>GSSGAFEDRDPTQFEERHLKFLQQLGKGNFGSVEMCRYDPLQDNTGEVVAVKKLQHSTEEHLRDFEREIEILKSLQHDNIVKYKGVCYSAGRRNLKLIMEYLPYGSLRDYLQKHKERIDHIKLLQYTSQICKGMEYLGTKRYIHRDLATRNILVENENRVKIGDFGL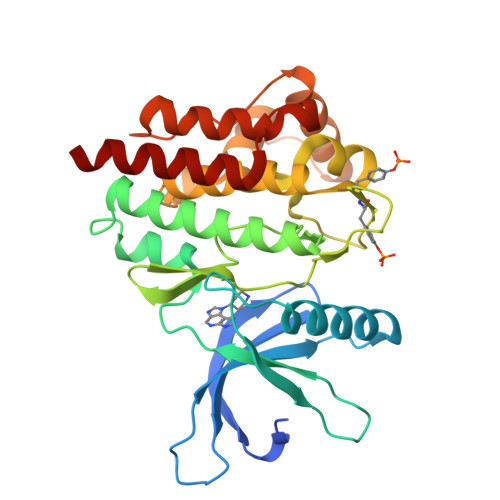TKVLPQDKEYYKVKEPGESPIFWYAPESLTESKFSVASDVWSFGVVLYELFTYIEKSKSPPAEFMRMIGNDKQGQMIVFHLIELLKNNGRLPRPDGCPDEIYMIMTECWNNNVNQRPSFRDLALRVDQIRDNMAG[2x]> ER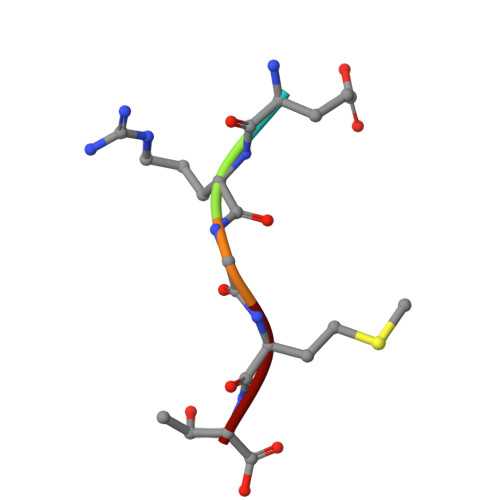GMT(2~{R})-4-[6-[4-[1-(hydroxymethyl)cyclopropyl]buta-1,3-diynyl]-3-oxidanylidene-1~{H}-pyrrolo[1,2-c]imidazol-2-yl]-2-methyl-2-methylsulfonyl-~{N}-oxidanyl-butanamide 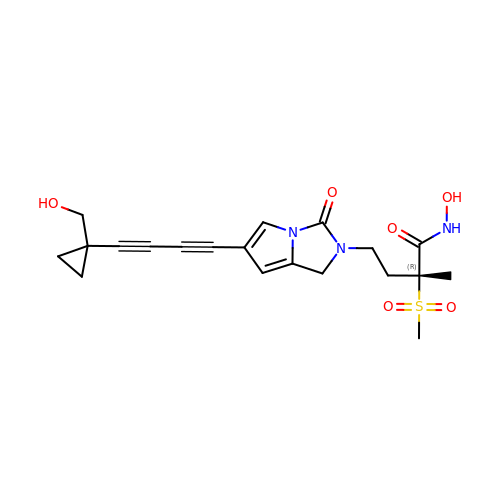| C20 H23 N3 O6 S | ROJCZRUQKASCDT-LJQANCHMSA-N>[2x]QSASQFTDPTTGFQFTGITDPVHDVTYGFVF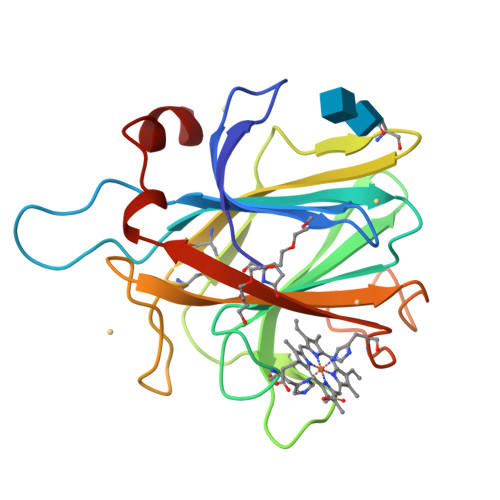PPLATSGAQSTEFIGEVVAPIASKWIGIALGGAHNNDLLLVAWANGNQIVSSTRWATGYVQPTAYTGTATLTTLPETTINSTHWKWVFRCQGCTEWNNGGGIDVTSQGVLAWAFSNVAVDDPSDPQSTFSEHTDFGFFGIDYSTAHSANYQNYLN>[2x]MGSSHHHHHHSQDPNSMGAFAKEEHQFLAELGLAQRNPGAFACGAWGGSGPTVTSTSPTNNQVIAEVVEASVHDYEEGMRACFDAAKTWMAIPAPKRGEIVRQIGDALRAKLHHLGRLVSLEMGKILPEGIGEVQEIIDMCDYAVGLSRQLNGSIIPSERPNHMMMEVWNPLGVVGVITAF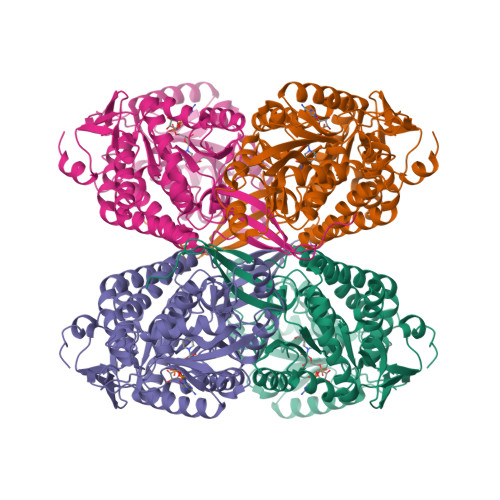NFPCAVLGWNACIALVCGNCVVWKGAPTTPLITIAMTKIVASVLEKNNLPGAIFTSFCGGTEIGQAIALDIRIPLVSFTGSTRAGLMVQQQVSARFGKCLLELSGNNAIIVMDDADIQLAVRSVLFAAVGTAGQRCTTCRRLILHENIYQTFLDQLVEVYKQVRIGDPLEKGTLLGPLHTPASKENFLKGIQTIKSQGGKILFGGSAIESEGNFVQPTIVEITPSAPVVKEELFGPVLYVMKFQTLKEAIEINNSVPQGLSSSIFTKRPDIIFKWLGPHGSDCGIVNVNIPTNGAEIGGAFGGEKATGGGREAGSDSWKQYMRRATCTINYGSELPLAQGINFG> MKKSLIALTLAALPVAAMADVTLYGTIKAGVETSRSVAHHGAQADRVKTATEIADLGSKIGFKGQEDLGNGLKAIWQLEQKAYVSGTDTGWGNRQSFIGLKGGFGKVRVGRLNNILKDTGNFNPWE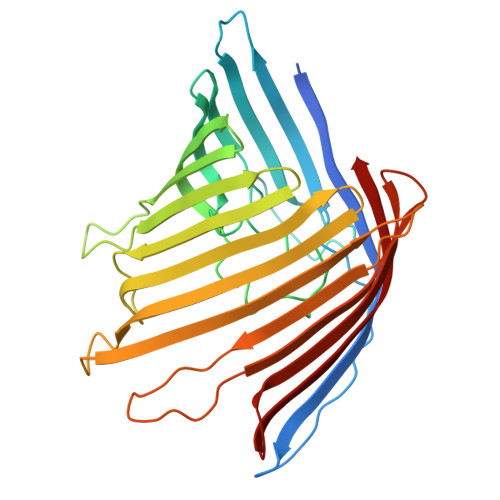GKSYYSGLSNIAQPEERHVSVRYDSPEFAGFSGSVQYVPNDNSGKNRSESYHAGFNYKNDGFFVQYAGSYKRHNYTTEKHQVHRLVGGYDHDALYASVAVQQQDAKLTWRDDNSHNSQTEVATTVAYRFGNVTPRVSYAHGFKGSVYDADHDNTYDQVVVGAEYDFSKRTSALVSAGWLQKGKGAEKFVATVGGVGLRHKF Our group previously produced a promiscuous designer enzyme by incorporating the noncanonical amino acid para-aminophenylalanine at position valine-15 of the Lactococcal multidrug resistance regulatory (LmrR) protein scaffold. In doing so, we enabled the formation of iminium ion intermediates formed by the condensation of aldehydes with the amino moiety of the pAF catalytic residue, thus mimicking known reactivities of small molecule organocatalysts in a protein scaffold. Assessment of the Michaelis–Menten kinetic parameters of these evolved mutants revealed that the mutations that improved one catalytic activity caused a concomitant decrease in the other, i.e., directed evolution produced catalytic specialization. We successfully obtained crystals for both the RGN and RMH mutants, with one crystal diffracting to a maximum resolution of 2.45 Å for the former mutant and two crystals diffracting at 2.55 and 2.24 Å for the latter.

However, RMH has new side chains installed proximal to the pAF residue. While in both crystal structures, the mutated M19 and H93 residues are close to the reactive amino moiety of the pAF residue, the R92 side chain conformer varies significantly. In crystal 2, the side chain points to the back of the pocket in both monomers, whereas in one monomer in crystal 1, it comes near the pAF-amino moiety. We hypothesized that the R92 and H93 side chains introduced in the evolved RMH variant could assist with formation and dehydration of the hemiaminal intermediate by acting as a H-bond donor and proton-shuttle, respectively. We used DFT to locate transition states and intermediates for a reaction pathway where H93 acts as a general-acid residue to promote hemiaminal formation and dehydration. With the participation of both H93 and R92 (i.e., the front-facing conformer), the reaction proceeds preferentially via the (S)-configured hemiaminal, with the highest overall barrier for this reaction sequence being the hemiaminal formation 15.2 kcal/mol above the lowest energy substrate conformer, and the dehydration step proceeding with a barrier of 8.7 kcal/mol (Figure 6B – green). Noncovalent interaction (NCI) analysis on the transition state structures was also conducted for both the forward- and backward-facing R92 conformations in the (S)-configured pathway to identify which NCIs may explain the role of R92 in lowering the transition-state energy.44 This analysis identified a hydrogen-bonding interaction between R92 and the hemiaminal-oxo moiety in the forward-facing conformation, which is not present in the backward-facing pathway. Our previous MD studies of the RMH-variant substrate-free resting state demonstrated that the motion of the two R92 side chains in each monomer is sensitive to mutations, with the cis-forward conformation (i.e., both R92 and R92’ facing toward the respective pAF15 residues) being greatly diminished in improved mutants.

>GAEIPKEMLRAQTNXILLMVLKQGDNYVYGIIKQVKEASNGEMELNEATLYTIFKRLEKDGIISSYWGDESQGGRRKYYRLTEIGHENMRLRHESWSRVDKIIENLEANKKSEAIKSRGGSGGWSHPQFEK[2x]> MTSTFDRVATIIAETCDIPRETITPESHAIDDLGIDSLDFLDIAFAIDKAFGIKLPLEKWTQEVNDGKATTEQYFVLKNLAARID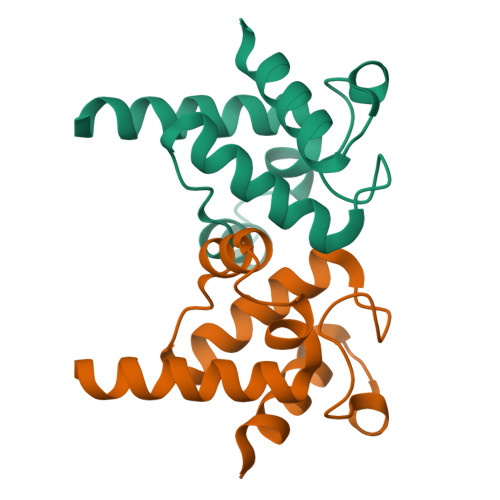ELVAAKGALEHHHHHH> HHHHHHDITFRNIRFRYKPDSPVILDNINLSIKQGEVIGIVGRSGSGKSTLTKLIQRFYIPENGQVLIDGHDLALADPNWLRRQVGVVLQDNVLLNRSIIDNISLANPGMSVEKVIYAAKLAGAHDFISELREGYNTIVGEQGAGLSGGQRQRIAIARALVNNPKILIFDEATSALDYESEHVIMRNMHKICKGRTVIIIAHRLSTVKNADRIIVMEK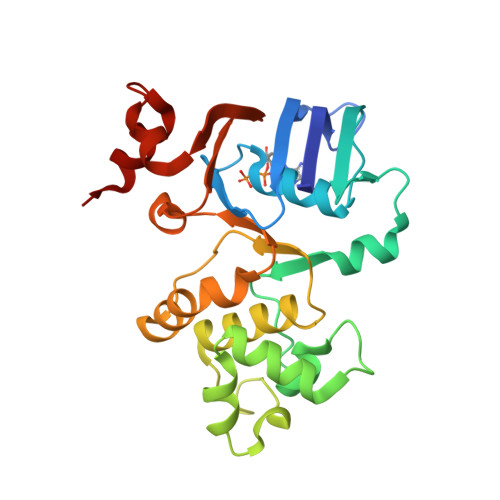GKIVEQGKHKELLSEPESLYSYLYQLQSD>[2x]SNASKMSDVKCTSVVLLSVLQQLRVESSSKLWAQCVQLHNDILLAKDTTEAFEKMVSLLSVLLSMQGAVDINKLCEEMLDNRATLQ;>[2x]EDKRAKVTSAMQTMLFTMLRKLDNDALNNIINNARDGCVPLNIIPLTTAAKLMVVIPDYNTYKNTCDGTTFTYASALWEIQQVVDADSKIVQLSEISMDNSPNLAWPLIVTALRANSAVKLQ

SARS-CoV-2 RdRp, also referred to as nonstructural protein 12 (Nsp12), is the catalytic center of the macromolecular complex frequently referred to as the replication transcription complex (RTC). The RTC is essential for virus replication because it makes copies of genomic and subgenomic RNAs and polymerizes antisense RNA. In SARS-CoV-2, besides RdRp (Nsp12), the RTC involves nonstructural proteins Nsp7, Nsp8, and others. Nsp12 is the largest component of the complex, and Nsp7 and Nsp8 are considered cofactors.

To provide insights into the structures, key residues of association, and multimeric state between the SARS-CoV-2 RTC’s cofactors, we solved high-resolution crystal structures of Nsp7 bound to Nsp8. The other structures were obtained from crystallization in the presence of protease Glu-C (V8). The C-terminus of the Nsp8 is well defined in Nsp7/8B, but not in other forms. In all of our crystal forms, the heterodimer formed between Nsp7 and 8 places Nsp7 near the half β-barrel-like domain of Nsp8 with the N-terminal helix of Nsp8 extended and pointing away (approximate dimensions of 40 × 40 × 46 Å). The similarity between all heterodimers in all our crystal forms is remarkable, with a root mean square deviation of 0.82 Å for 184 aligned Cα atoms despite different unit cell dimensions, different space groups, and different asymmetric units. In contrast to previously reported Nsp7/8 structures from other coronaviruses, in all three of our structures, either as in the asymmetric content or symmetry related, a heterotetramer or a dimer of heterodimers is present as an elongated, thick rod shape of 40 × 92 Å. The differing crystal forms show only slight variation in the packing of Nsp7/8 heterodimers to form heterotetramers. The heterotetramers are formed between the two heterodimers that are related by the noncrystallographic twofold rotational symmetry. Comparing the heterotetramers in the asymmetric units, the RMSD is 1.28 Å for 368 aligned Cα atoms.>MAQFDTEYQRLEASYSDSPPGEEDLLVHVAEGSKSPWHHIE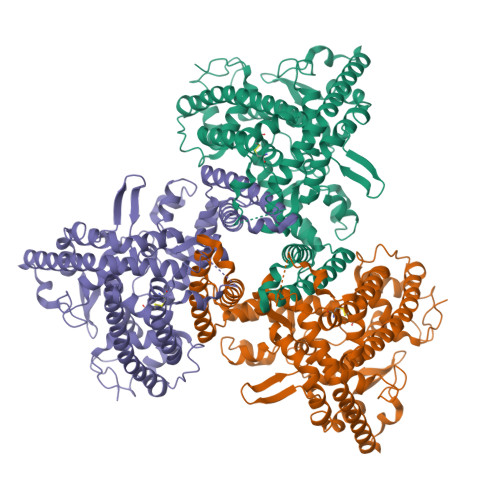NLDLFFSRVYNLHQKNGFTCMLIGEIFELMQFLFVVAFTTFLVSCVDYDILFANKMVNHSLHPTEPVKVTLPDAFLPAQVCSARIQENGSLITILVIAGVFWIHRLIKFIYNICCYWEIHSFYLHALRIPMSALPYCTWQEVQARIVQTQKEHQICIHKRELTELDIYHRILRFQNYMVALVNKSLLPLRFRLPGLGEAVFFTRGLKYNFELILFWGPGSLFLNEWSLKAEYKRGGQRLELAQRLSNRILWIGIANFLLCPLILIWQILYAFFSYAEVLKREPGALGARCWSLYGRCYLRHFNELEHELQSRLNRGYKPASKYMNCFLSPLLTLLAKNGAFFAGSILAVLIALTIYDEDVLAVEHVLTTVTLLGVTVTVCRSFIPDQHMVFCPEQLLRVILAHIHYMPDHWQGNAHRSQTRDEFAQLFQYKAVFILEELLSPIVTPLILIFCLRPRALEIIDFFRNFTVEVVGVGDTCSFAQMDVRQHGHPQWLSAGQTEASVYQQAEDGKTELSLMHFAITNPGWQPPRESTAFLG[3x]> MSKVPRNFRLLEELEKGEKGFGPESCSYGLADSDDITMTKWNGTILGPPHSNHENRIYSLSIDCGPNY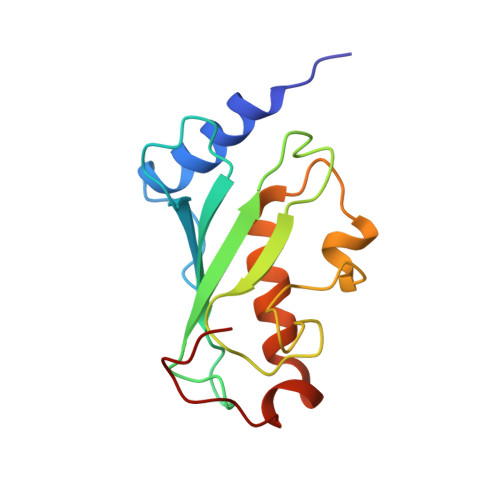PDSPPKVTFISKINLPCVNPTTGEVQTDFHTLRDWKRAYTMETLLLDLRKEMATPANKKLRQPKEGETF>MTMEKGMSSGEGLPSRSSQVSAGKITAKELETKQSYKEKRGGFVLVHAGAGYHSESKAKEYKHVCKRACQKAIEKLQAGALATDAVTAALVELEDSPFTNAGMGSNLNLLGEIECDASIMDGKSLNFGAVGALSGIKNPVSVANRLLCEGQKGKLSAGRIPPCFLVGEGAYRWAVDHGIPSCPPNIMTTRFSLAAFKRNKRKLELAERVDTDFMQLKKRRQSSEKENDSGTLDTVGAVVVDHEGNVAAAVSSGGLALKHPGRVGQAALYGCGCWAENTGAHNPYSTAVSTSGCGEHLVRTILARECSHALQAEDAHQ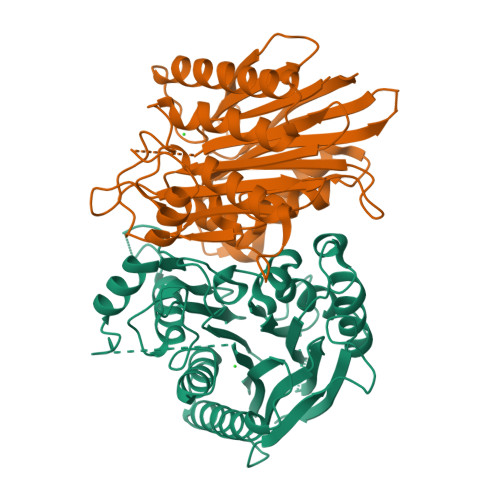ALLETMQNKFISSPFLASEDGVLGGVIVLRSCRCSAEPDSSQNKQTLLVEFLWSHTTESMCVGYMSAQDGKAKTHISRLPPGAVAGQSVAIEGGVCRLESPVN[2x]> AGEARLEEAVNRWVLKFYFHEALRAFRGSRYGDFRQIRDIMQALLVRPL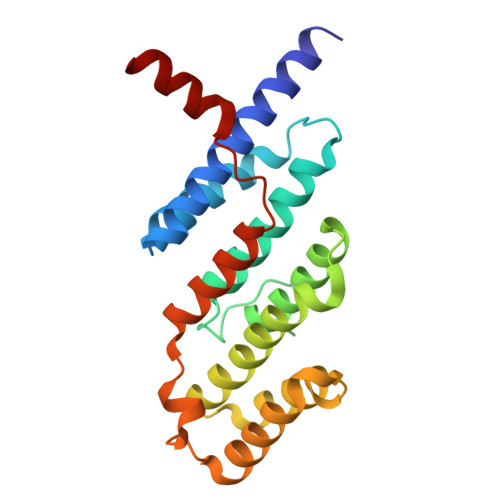GKEHTVSRLLRVMQCLSRIEEGENLDCSFDMEAELTPLESAINVLEMIKTEFTLTEAVVESSRKLVKEAAVIICIKNKEFEKASKILKKHMSKDPTTQKLRNDLLNIIREKNLAHPVIQNFSYETFQQKMLRFLESHLDDAEPYLLTMAKKALK>[2x]GAMGSSLDNPTPFPNLGPSENPLKRLLVPGEEWEFEVTAFYRGRQVFQQTISCPEGLRLVGSEVGDRTLPGWPVTLPDPGMSLTDRGVMSYVRHVLSCLGGGLALWRAGQWLWAQRLGHCHTYWAV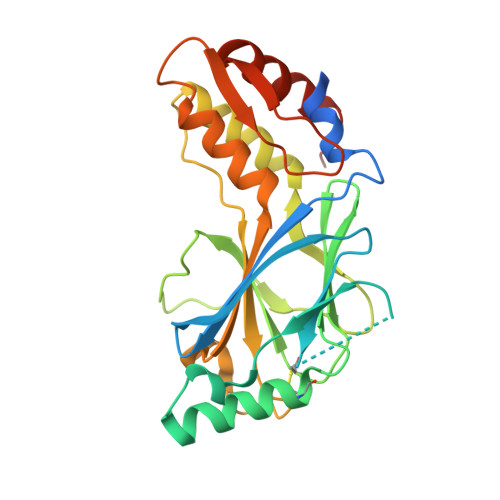SEELLPNSGHGPDGEVPKDKEGGVFDLGPFIVDLITFTEGSGRSPRYALWFCVGESWPQDQPWTKRLVMVKVVPTCLRALVEMARVGGASSLENTVDLHISNSHPLSLTSDQYKAYLQDLVEGMDFQGPGES>GSHMEDYNFVFKVVLIGESGVGKTNLLSRFTRNEFSHDSRTTIGVEFSTRTVMLGTAAVKAQIWDTAGLERYRAITSAYYRGAVGALLVFDLTKHQTYAVVERWLKELYDHAEATIVVMLVGNKSDLSQAREVPTEEARMFAENNGLLFLETSALDSTNVELAFETVLKEIFAKVSKQ[2x]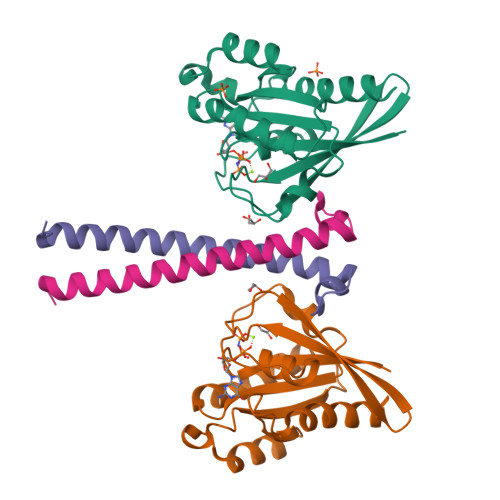;>SMNPFDATAGYRSLTYEEVLQELVKHKELLRRKDTHIRELEDYIDNLLVRVMEETPSILRVPYEPSRKAGKFSNS[2x]>[4x]GIDPFTQRERARQID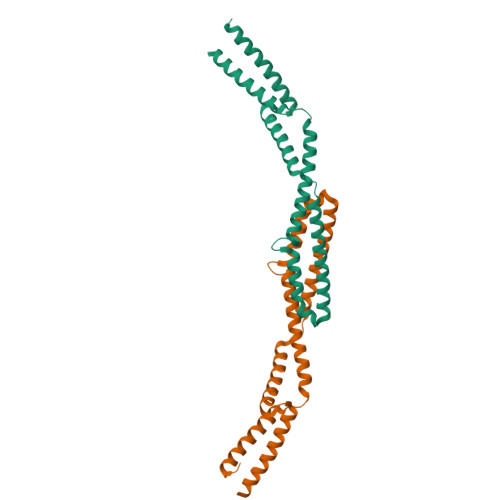LLAFQVQEISEVSPDPGEEEGLNTELSRLSNLHTIAQAAAGGVELLSDGDLNAAGLIGEAVRALNAGAKYDETVMQLQNELRAALESVQAIAGELRDVAEGSAADPEALDRVEARLSALSKLKNKYGPTLEDVVEFGAQAAEELAGLEEDERDAGSLQAD OmCI is a bifunctional protein derived from blood-feeding ticks that specifically prevents complement (C)-mediated C5 activation and also sequesters leukotriene B4 (LTB4) within an internal binding pocket. The 17-kDa lipocalin Ornithodoros moubata complement inhibitor OmCI, originally isolated from an ectoparasitic tick (Acari), is a bifunctional protein that may have such therapeutic advantages. By binding directly to C5 in the vicinity of the C5-C345C domain OmCI prevents cleavage of C5 by the C5 complement convertases, thereby preventing release of anaphylatoxin C5a and formation of the terminal 5b-9 C complex (TCC). We describe two crystal structures of bacterially expressed OmCI: one binding a C16 fatty acid and the other binding LTB4 (C20).

The ligands are also of different lengths (C16, C18, and C20, respectively, for palmitoleic acid, ricinoleic acid, and LTB4); LTB4 fills the pocket completely, whereas the yOmCI-ricinoleic acid and bOmCI-palmitoleic acid complexes show a water molecule filling the bottom of the pocket. Hydroxylation at this position is common to ricinoleic acid and LTB4, and both complexes show the -OH group on C12 forming hydrogen bonds to His-119 and Asp-121. Gln-105 recognizes the -OH at LTB4 C5. The C9=C10 double bond present in LTB4, but not in palmitoleic or ricinoleic acid, stacks against the guanidinium head of Arg-107. The same Arg side chain is the source of the selectivity against cyclic eicosanoids such as TXB2 and TXA2 (43), as it makes the pocket too narrow to accommodate cyclic ligands. The hydrophobic side chains of Phe-36, Tyr-43, Leu-57, Gly-59, Pro-61, Leu-70, Val-72, Met-74, Phe-76, Trp-87, Phe-89, Arg-107, and Trp-133 contact the hydrophobic body of all three ligands. The three ligands all bind with their carboxylic acid head at the solvent-exposed brim of the OmCI pocket, hydrogen bonding to the side chains of Arg-54, Thr-85, and Trp-87. The other main locus of structural variability in the bOmCI and yOmCI structures is the conformation of the βH-α3 loop (amino acids 132–142), shown previously to be required for C5 inhibition, which in both complexes of bOmCI swings inward, with the concomitant flip of the side chain of His-117. Dispersion interactions between the conjugated leukotriene and nearby amino acids cause the shift, which is consistent with the triene chromophore of LTB4 being completely encompassed by OmCI.

>[4x]DSESDCTGSEPVDAFQAFSEGKEAYVLVRSTDPKARDCLKGEPAGEKQDNTLPVMMTFKNGTDWASTDWTFTLDGAKVTATLGNLTQNREVVYDSQSHHCHVDKVEKEVPDYEMWMLDAGGLEVEVECCRQKLEELASGRNQMYPHLKDC Flavodoxins (Flds), which are electron-carrier flavoproteins of small molecular mass that contain FMN as the prosthetic group, are found in various microorganisms, and play multiple roles in varied pathways. Flds generally contain one non-covalently bound FMN that acts as an electron-transfer center by switching three redox states, including the hydroquinone, semiquinone and oxidized states. Flds in Desulfovibrio sp. are suggested to participate in two major reactions as shown in the scheme below; the dashed lines represent other proteins participating in the reactions. In the present work, we isolated a native functional “short-chain” Fld containing 146 amino acids with the cofactor FMN directly from anaerobically grown D. gigas cells.

We report here the structure of the short-chain Fld from D. gigas at a resolution of 1.3 Å; we study its structural-functional relationship and the prospective binding region for an electron-transferring partner. The results show that the structure of Fld from D. gigas is a dimer containing two FMN molecules with the monomers orientated head to head, which agrees with the solution state. The electrostatic surface of the FMN-binding pocket reveals that the binding site for FMN is hydrophobic with aromatic residues, e.g., Trp60 and Phe101, whereas the binding pocket for the phosphate group is positively charged. The isoalloxazine ring of FMN was stabilized with loops Asp95–Gly103 and Thr59–Asp63, in which Trp60 and Tyr98 located at both sides of the isoalloxazine ring are the most important for providing direct π-π interactions. The amino acids from Ser10 to Thr15 form a loop that provides several hydrogen bonds to stabilize the phosphate group of FMN. Superimposing the structures of the two monomers in the Fld dimer reveals a small r.m.s. deviation (0.37 Å), implying that the overall folding of each of the monomers is similar, but a detailed inspection of the conformation shows that the structures and positions of some main chains and the co-factors are notably altered, especially a conformational alteration around the active site. This comparison showed that two FMN-coordination loops (Thr59–Asp63 and Ser96–Thr99) are not at the same corresponding position in the two monomers, in which Asp63 and Tyr98 exhibit the largest vibration distances ~6.2 and 1.5 Å, respectively. The peptide of Gly61 points to atom N5 of FMN with distances 3.7 and 3.6 Å, respectively, in monomers A and B. However, the structure and character of FMN are easily affected by X-ray radiation damage. The interface of dimerization notably contains no charge or slight positive charge distribution; dimerization hence exposes and creates a more negatively charged environment on the surface of the Fld dimer by concealing the uncharged or positively charged residues at the dimeric interface.

>[2x]MPKALIVYGSTTGNTEGVAEAIAKTLNSEGMETTVVNVADVTAPGLAEGYDVVLLGCSTWGDDEIELQEDFVPLYEDLDRAGLKDKKVGVFGCGDSSYTYFCGAVDVIEKKAEELGATLVASSLKIDGEPDSAEVLDWAREVLARV>MIIGNNLHVDAFYDEATSTISYLVMDRETRQCALIDSVLDYDPKSGRTCSASADRLVERVNELNASVRWVLETHVHADHLSAAAYLKEKLGGHTAIGAHITQVQKVFGALFNAEPGFARDGSQFDVLLEDEEGFRIGNLQARALHTPGHTPACMSFMIEDAGEIAVFVGDTLFMPDYGTARCDFPGADARTLYRSIRRLLAFPDQTRLFMCHDYLPGGRDMQYVTTVAEQ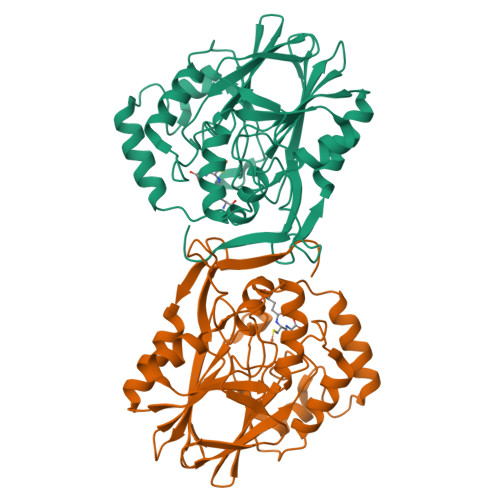RASNIHIHQGIDEDSFVAMREARDKTLEMPVLILPSVQVNMRSGQLPPPEANGVSYLKIPLNKL[2x]(2Z)-2-(1H-1,2,4-triazol-1-yl)-3-[3-(3,4,5-trimethoxyphenyl)-1H-indazol-5-yl]prop-2-enenitrile 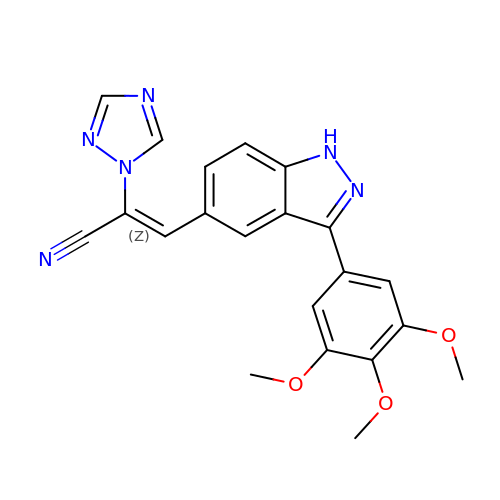| C21 H18 N6 O3 | KVQZHZNPPJMLLH-UHFFFAOYSA-N> SMVEDHYEMGEELGSGQFAIVRKCRQKGTGKEYAAKFIKKRRLSSSRRGVSREEIEREVNILREIRHPNIITLHDIFENKTDVVLILELVSGGELFDFLAEKESLTEDEATQFLKQILDGVHYLHSKRIAHFDLKPENIMLLDKNVPNPRIKLIDFGIAHK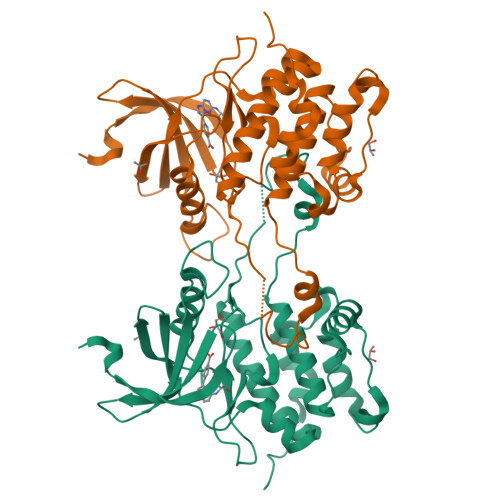IEAGNEFKNIFGTPEFVAPEIVNYEPLGLEADMWSIGVITYILLSGASPFLGETKQETLTNISAVNYDFDEEYFSNTSELAKDFIRRLLVKDPKRRMTIAQSLEHSWIKAIRRRNVRGEDSG>MLKLQTLQALICIEEVGSLRAAAQLLHLSQPALSAAIQQLEDELKAPLLVRTKRGVSLTSFGQAFMKHARLIVTESRRAQEEIGQLRGRWEGHITFAASPAIALAALPLALASFAREFPDVTVNVRDGMYPAVSPQLRDGTLDFALTAAHKHDIDTDLEAQPLYVSDVVIVGQRQHPMANATRLAELQECRWAFSSAPRGPGAIIRNAFARYGLPEPKLGLVCESFLALPGVVAHSDLLTTMPRTLYERNAFKDQLCSIPLQDALPNPTIYVLRRHDLPVTPAAAGLIRWIQHHALQ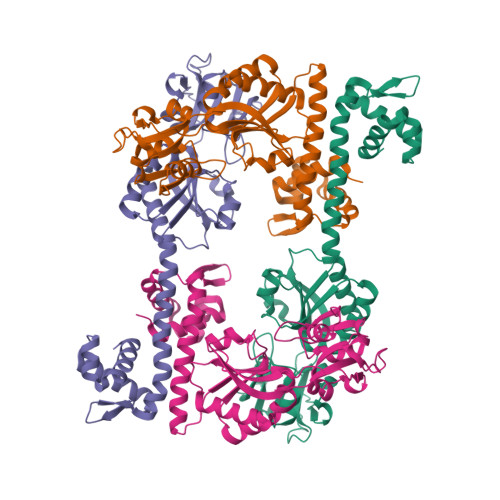TGHHHHHH[10x]>[2x]MMSDQENENEHAKAFLGLAKCEEEVDAIEREVELYRLNKMKPVYEKRDAYIDEIAEFWKIVLSQHVSFANYIRASDFKYIDTIDKIKVEWLALESEMYDTRDFSITFHFHGIEGDFKEQQVTKVFQIKKGKDDQEDGILTSEPVPIEWPQSYDSINPDLIKDKR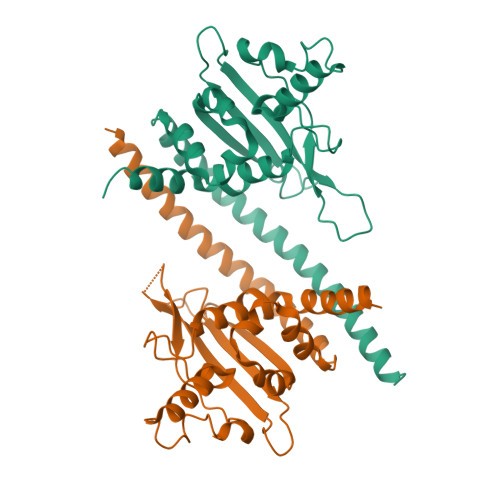SPEGKKKYRQGMKTIFGWFRWTGLKPGKEFPHGDSLASLFSEEIYPFCVKYYAEAQRDLEDEEGESGLSADGDSEDDDGSLGEVDLPLSDEEPSSKKRKV;> EVDLPLSDEEPSS> RLKGKVKWFNSEKGFGFIEVEGQDDVFVHFSAIQG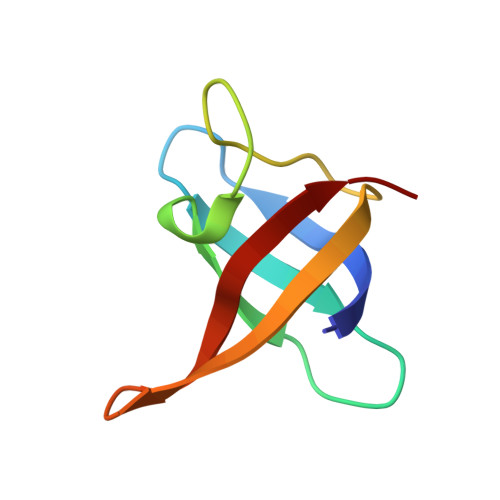EGFKTLEEGQAVSFEIVEGNRGPQAANVTIEA> DYVLYKDATKPVEDRVADLLGRMTLAEKIGQMTQIERLVATPDVLRDNFIGSLLSGGGSVPR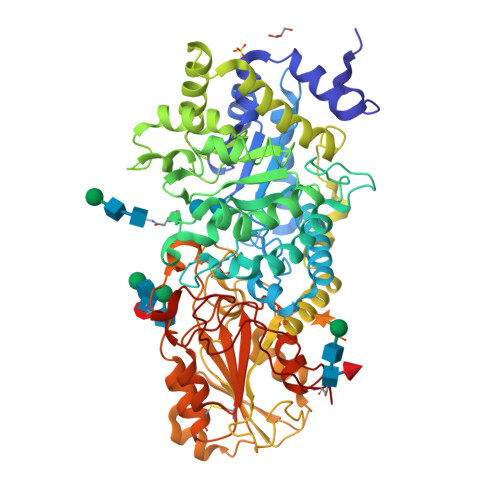KGATAKEWQDMVDGFQKACMSTRLGIPMIYGIDAVHGQNNVYGATIFPHNVGLGATRDPYLVKRIGEATALEVRATGIQYAFAPCIAVCRDPRWGRCYESYSEDRRIVQSMTELIPGLQGDVPKDFTSGMPFVAGKNKVAACAKHFVGDGGTVDGINENNTIINREGLMNIHMPAYKNAMDKGVSTVMISYSSWNGVKMHANQDLVTGYLKDTLKFKGFVISDWEGIDRITTPAGSDYSYSVKASILAGLDMIMVPNKYQQFISILTGHVNGGVIPMSRIDDAVTRILRVKFTMGLFENPYADPAMAEQLGKQEHRDLAREAARKSLVLLKNGKTSTDAPLLPLPKKAPKILVAGSHADNLGYQCGGWTIEWQGDTGRTTVGTTILEAVKAAVDPSTVVVFAENPDAEFVKSGGFSYAIVAVGEHPYTETKGDNLNLTIPEPGLSTVQAVCGGVRCATVLISGRPVVVQPLLAASDALVAAWLPGSEGQGVTDALFGDFGFTGRLPRTWFKSVDQLPMNVGDAHYDPLFRLGYGLTTNATKKY[(2R,3S,4R,5R)-5-(6-amino-9H-purin-9-yl)-3,4-dihydroxytetrahydrofuran-2-yl]methyl (3R)-4-[(3-{[2-(ethylsulfanyl)ethyl]amino}-3-oxopropyl)amino]-3-hydroxy-2,2-dimethyl-4-oxobutyl 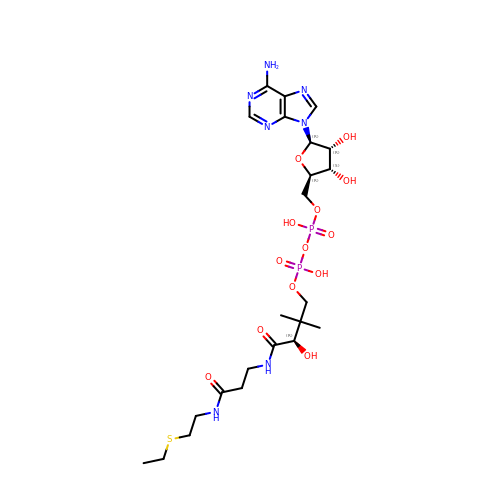dihydrogen diphosphate (non-preferred name) | C23 H39 N7 O13 P2 S | ZYQGAGMIMDQCKA-ZSJPKINUSA-N> MGCTLSAEDKAAVERSKMIDRNLREDGERSARLVKILLLGAGESGKSTFLKQMRIIHGQDFDQRAREEFRPTIYSNVIKGMRVLVDAREKLHIPWGDNKNQLHGDKLMAFDTRAPMAAQGMVETRVFLQYLPAIRALWEDSGIQNAYDRRREFQLGESVKYFLDNLDKLGVPDYIPSQQDILLARRPTKGIHEYDFEIKNVPFKMVDVGGQRSERKRWFECFDSVTSILFLVSSSEFDQVLMEDRQTNRLTESLNIFETIVNNRVFSNVSIILFLNKTDLLEEKVQVVSIKDYFLEFEGDPHCLRDVQKFLVE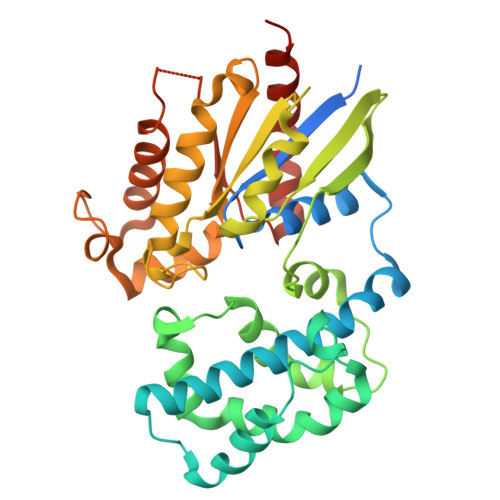CFRGKRRDQQQRPLYHHFTTAINTENIRLVFRDVKDTILHDNLKQLMLQ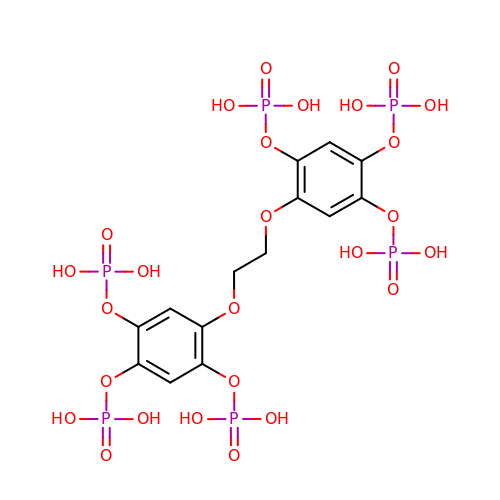5,5'-(ethane-1,2-diylbis(oxy))bis(benzene-5,4,2,1,-tetrayl)hexakisphosphate | C14 H20 O26 P6 | SPZGMBGXCYAMCB-UHFFFAOYSA-N> EQQRFPQRYIELAIVVDHGMYTKYSSNFKKIRKRVHQMVSNINEMCRPLNIAITLALLDVWSEKDFITVQADAPTTAGLFGDWRERVLLKKKNHDHAQLLTDTNFARNTIGWAYVGRMCDEKYSVAVVKDHSSKVFMVAVTMTHELGHNLGMEHDDKDKCKCDTCIMSAVISDKQSKLFSDCS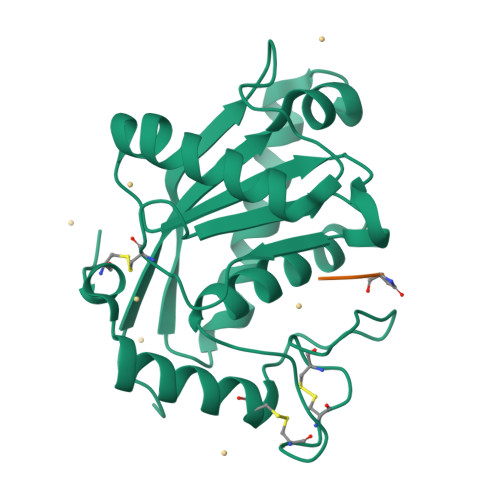KDYYQTFLTNDNPQCILNAP;> QQW> EVRLSVPPLVEV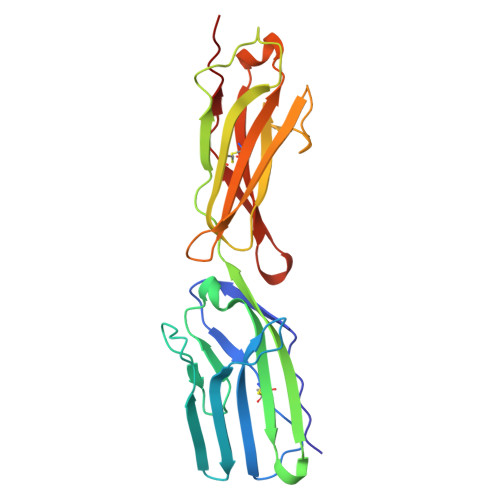MRGKSVILDCTPTGTHDHYMLEWFLTDRSGARPRLASAEMQGSELQVTMHDTRGRSPPYQLDSQGRLVLAEAQVGDERDYVCVVRAGAAGTAEATARLNVFAKPEATEVSPNKGTLSVMEDSAQEIATCNSRNGNPAPKITWYRNGQRLEVPVEMNPEGYMTSRTVREASGLLSLTSTLYLRLRKDDRDASFHCAAHYSLPEGRHGRLDSPTFHLTLHY> GAMGMSSLQKRPGPGNSSQPTERPRKESILDLSRYQDQRIQATFTGGRQITGIL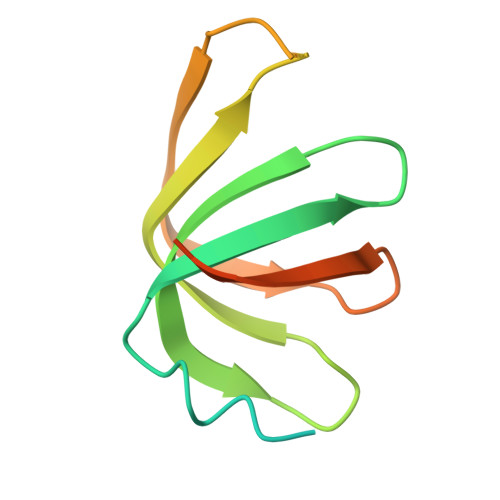KGFDQLMNLVLDDVEEQLRNPEDGKLTGAIRKLGLVVVRGTTLVLIAPMDGSEEIPNPFVQAE> VFEWFGSNESGAEFGTNIPGVWGTDYIFPDPSAISTLIDKGMNFFRVQFMMERLLPDSMTGSYDEEYLANLTTVIKAVTDGGAHALVDPHNYGRYNG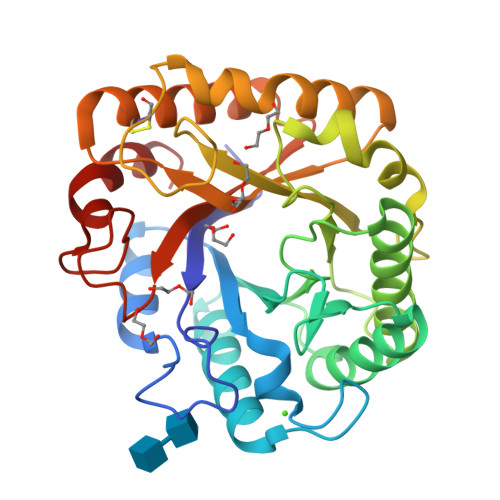EIISSTSDFQTFWENLAGQYKDNDLVMFDTNNEYHDMDQDLVLNLNQAAINGIRAAGATSQYIFVEGNSWTGAWTWVDVNDNMKNLTDPEDKIVYEMHQYLDSDGSGTSETCVSETIGKERVTEATQWLKDNKKVGFIGEYAGGSNDVCRSAVSGMLEYMANNTDVWKGASWWAAGPWWGDYIFSLEPPDGTAYTGMLDILEAYL> ASKAAAPPPVRLFGVEGTYATALYQAAAKNS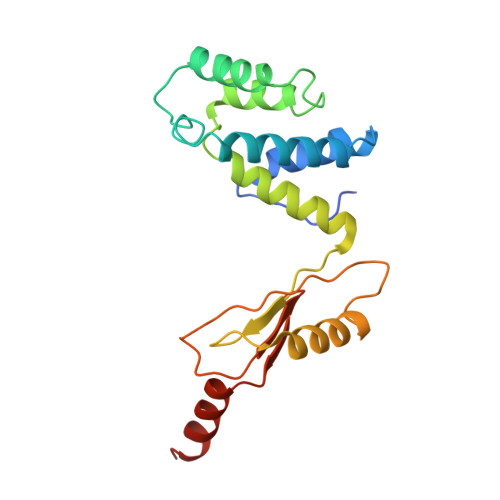SIDAAFQSLQKVESTVKKNPKLGHLLLNPALSLKDRNSVIDAIVETHKNLDGYVVNLLKVLSENNRLGCFEKIASDFGVLNDAHNGLLKGTVTSAEPLDPKSFKRIEKALSASKLVGQGKSLKLENVVKPEIKGGLIVELGDKTVDLSISTKIQKLNKVLEDSI> DAAQPATEFAKSQDLPYQSLSIDTFSYLNDEYVVIAQPFTGKCIFLEWDHVEKTFRNYDNITGTSTVVCKPIVIETQLYVIVAQLFGGSHIYKRDSFANKFIKIQDIEILKIRKPNDIETFKIENNWYFVVADSSKAGFTTIYKWNGNGFYSHQSLHAWYRDTDVEYLEIVRTPQTLRTPHLILSSSSQRPVIYQWNKATQLFTNQTDIPNMEDVYAVKHFSVKGDVYICLTRFIG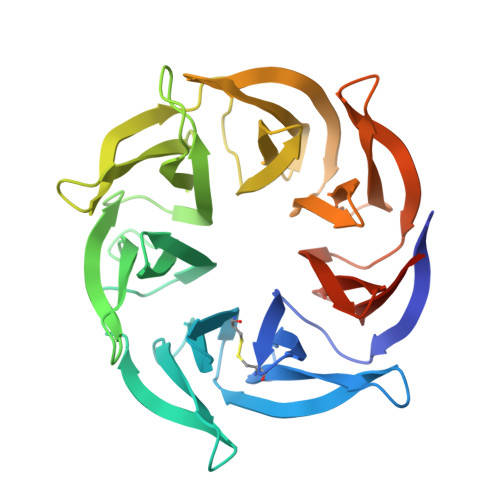DSKVMKWGGSSFQDIQRMPSRGSMVFQPLQINNYQYAILGSDYSFTQVYNWDAEKAKFVKFQELNVQAPRSFTHVSINKRNFLFASSFKGNTQIYKHVIVDLSAKHHHHHH>GILDPEERYEHQLRQLNDMGF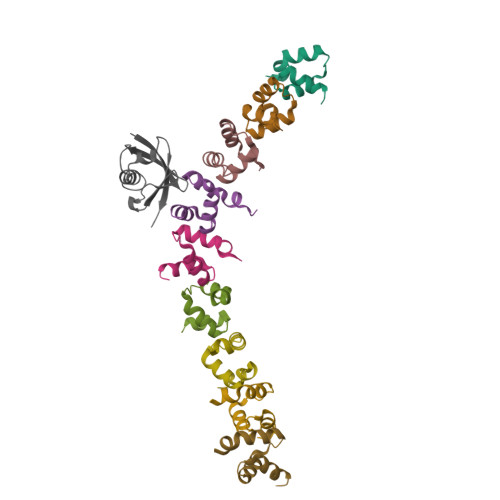FDFDRNVAALRRSGGSVQGALDSLLNGDV[18x];>LDMSLNIHIKSGQDKWEVNVAPESTVLQFKEAINKANGIPVANQRLIYSGKILKDDQTVESYHIQDGHSVHLVKSQP[3x]>MQRGSAYFLRGRARQNLKVLLLYCAFLLVMLLAYASIFRYLMWHLEGRAYSFMAGIYWTITVMTTLGFGDITFESDAGYLFASIVTVSGVIFLDIILPFGFVSMFLAPWIERRLRYHPTIELPDDTRGHILIFGIDPITRTLIRKLESRNHLFVVVTDNYDQALHLEEQEGFKVVYGSPTDAHVLAGLRVAAARSIIANLSDPDNANLCLTVRSLCQTPIIAVVKEPVHGELLRLAGANQVVPLTRILGRYLGIRATTCGALAHILDSFGNLQIAELPVHGTPFAGKTIGESGIRQRTGLSIIGVWERGSLTTPQRETVLTEQSLLVLAGTKSQLAALEYLIGEAPEDELIFIIGHGRIGCAAAAFLDRKPVPFILIDRQESPVCNDHVVVYGDATVGQTLRQAGIDRASGIIVTTNDDSTNIFLTLACRHLHSHIRIVARANGEENVDQLYAAGADFVVSNASVGANILGNLLEHKESAFLSEGMAVFRRPLPPAMAGKTIAETRLRPLTGCSIVAIEAPDRADILISPPPETILAEGARLILIGTSEQEKTFDQTIAARLVPR[4x]

Each GsuK subunit contains two tandem RCK domains, reminiscent of Slo K+ channels. We demonstrate that GsuK is a nucleotide-activated and Ca2+-deactivated K+ channel and reveal the structural mechanism of multi-ligand gating of this double-RCK K+ channel and a distinct pore opening mechanics. Ca2+ stabilizes the closed gating ring by binding at the inter-subunit assembly interfaces and deactivates the GsuK channel. While both NAD+ and ADP anchor their adenine rings at the same site on RCK2 by using the conserved nucleotide binding motif, they utilize different functional groups and activate the channel at different sites.

To reveal the structural basis of nucleotide activation, we also co-crystallized the L97D mutant with ADP and NAD+ and determined the complex structures at 2.8 and 3.2 Å, respectively. The overall structure of the nucleotide-bound L97D mutant is similar to that of the apo state, with the gating ring in a Ca2+-bound, closed conformation. In the ADP-bound structure, the AMP moiety of the ligand can be unambiguously defined in all four subunits within the asymmetric unit at the same position as was observed in the isolated gating ring structure. The electron density for the β-phosphate group, although not as well resolved as the rest due to higher mobility, points to two possible configurations. In one subunit, the ADP is in an extended trans configuration, whereas in the other subunits the ADP is in a cis configuration with respect to the phosphoester bond. In the cis configuration, the β-phosphate makes a sharp turn and inserts itself into a pocket formed by the loops from βA-to-αA and from βD-to-αD on the second RCK domain. The pocket is located at the base of the flexible interface and analogous to the Ca2+ binding site in the MthK RCK, suggesting that ADP binding in the cis configuration represents an activating state and promotes the gating ring conformational change at the flexible interface similar to Ca2+ binding in MthK. Albeit with opposite gating effect, the Ca2+ binding site of GsuK is analogous to the position of the Ca2+-bowl in BK; and the ADP activation site in GsuK is equivalent to the Ca2+ binding site in MthK.> MINQEKRPFRIRDKYIDRDSEYLLQENEPDATLDQQLLEDLQKKKTDLRYIEMQRFREKLPSYGMQKELVNMIDNHQVTVISGETGCGKTTQVTQFILDNYIERGKGSACRIVCTQPRRISAISVAERVAAERAESCGNGNSTGYQIRLQSRLPRKQGSILYCTTGIILQWLQSDPHLSSVSHIVLDEIHERNLQSDVLMTVVKDLLSYRPDLKVVLMSATLNAEKFSEYFGNCPMIHIPGFTFPVVEYLLEDIIEKIRYVPEQKEHRSQFKKGFMQGHVNRQEKYYYEAIYKERWPGYLRELRQRYSASTVDVVEMMDDEKVDLNLIAALIRYIVLEEEDGAILVFLPGWDNISTLHDLLMSQVMFKSDKFIIIPLHSLMPTVNQTQVFKRTPPGVRKIVIATNIAETSITIDDVVYVIDGGKIKETHFDTQNNISTMSAEWVSKANAKQRKGRAGRVQPGHCYHLYNSLRASLLDDYQLPEILRTPLEELCLQIKILRLGGIAHFLSRLMDPPSNEAVLLSIKHLMELNALDKQEELTPLGVHLARLPVEPHIGKMILFGALFCCLDPVLTIAASLSFKDPFVIPLGKEKVADARRKELAKDTKSDHLTVVNAFKGWEKAKQRGFRYEKDYCWEYFLSSNTLQMLHNMKGQFAEHLLGAGFVSSRNPQDPESNINSDNEKIIKAVICAGLYPKVAKIRLNLGKKRKMVKVYTKTDGVVAIHPKSVNVEQTEFNYNWLIYHLKMRTSSIYLYDCTEVSPYCLLFFGGDISIQKDNDQETIAVDEWIIFQSPARIAHL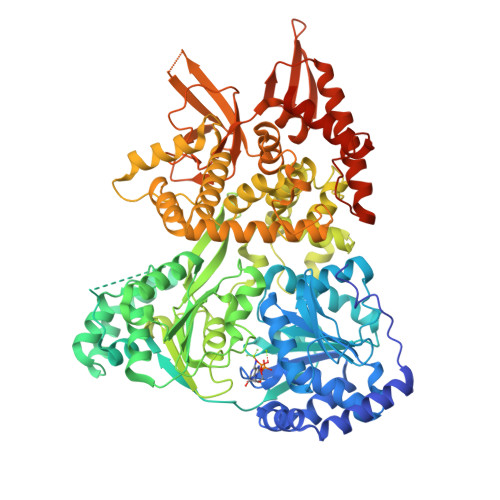VKELRKELDILLQEKIESPHPVDWKDTKSRDCAVLSAIIDLIKTQEKATPRNLPPRFQDGYYSPHHHHHHHH>FEARLVQGSILKKVLEALKDLINEACWDISSSGVNLQSMDSSHVSLVQLTLRSEGFDTYRCDRNLAMGVNLTSMSKILKCAGNEDIITLRAEDNADTLALVFEAPNQEKVSDYEMKLMDLDVEQLGIPEQEYSCVVKMPS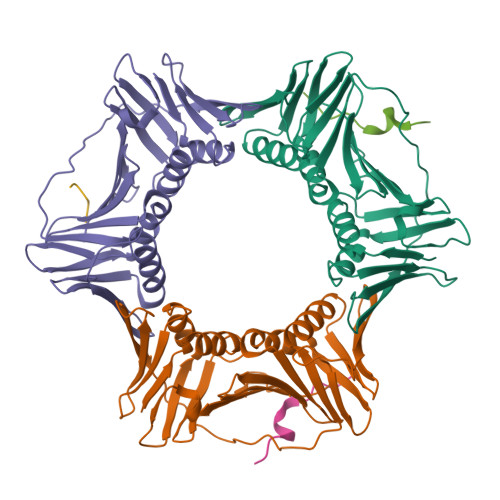GEFARICRDLSHIGDAVVISCAKDGVKFSASGELGNGNIKLSQTSNVDKEEEAVTIEMNEPVQLTFALRYLNFFTKATPLSSTVTLSMSADVPLVVEYKIADMGHLKYYLAPK[3x];>[2x]AFQAKLDTFLWS;> AGAGA>[2x]SGTATYSGNPFVGVTPWANAYYASEVSSLAIPSLTGAMATAAAAVAKVPSFMWLDTLDKTPLMEQTLADIRTANKNGGNYAGQFVVYDLPDRACAALASNGEYSIADGGVAKYKNYIDTIRQIVVEYSDIRTLLVIEPDSLANLVTNLGTPKCANAQSAYLECINYAVTQLNLPNVAMYLDAGHAGWLGWPANQDPAAQL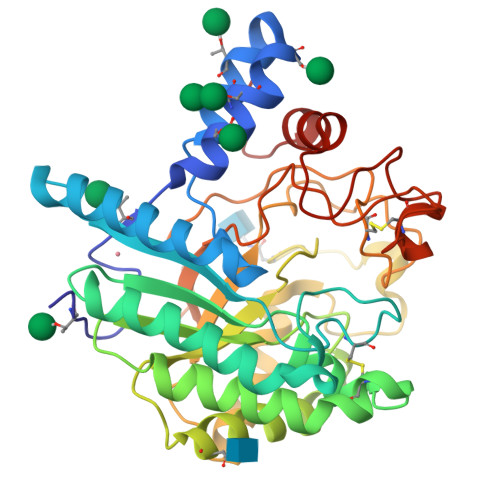FANVYKNASSPRALRGLATNVANYNGWNITSPPSYTQGNAVYNEKLYIHAIGPLLANHGWSNAFFITDQGRSGKQPTGQQQWGDWCNVIGTGFGIRPSANTGDSLLDSFVWVKPGGECDGTSDSSAPRFDSHCALPDALQPAPQAGAWFQAYFVQLLTNANPSFL>SANEDMPVEKILEAELAVEPKTETYVEANMGLNPSSPNDPVTNICQAADKQLFTLVEWAKRIPHFSELPLDDQVILLRAGWNELLIASFSHRSIAVKDGILLATGLHVHRNSAHSAGVGAIFDRVLTELVSKMRDMQMDKTELGCLRAIVLFNPDSKGLSNPAEVEALREKVYASLEAYCKHKYPEQPGRFAKLLLRLPALRSIGLKCLEHLFFFKLIGDTPIDTFLMEMLEAPHQAT[2x];>MSKESVRNDRNKKKKEPSKQECTESYEMTAELDDLTEKIRKAHQETFPSLCQLGKYTTNSSADHRVRLDLGLWDKFSELATKCI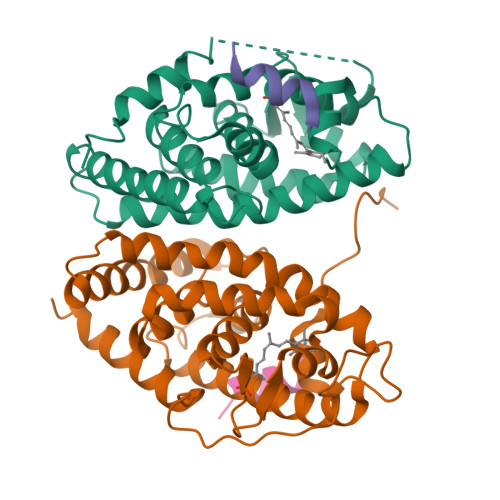IKIVEFAKRLPGFTGLTIADQITLLKAACLDILILRICTRYTPEQDTMTFSDGLTLNRTQMHNAGFGPLTDLVFTFANQLLPLEMDDTETGLLSAICLICGDRQDLEEPTKVDKLQEPLLEALKIYIRKRRPSKPHMFPKILMKITDLRSISAKGAERVITLKMEIPGSMPPLIQEMLENSEGHEPLTPSSSGNIAEHSPSVSPSSVENSGVSQSPLLQ[2x];>[4x]NHPMLMNLLKDNPA Here, we present InCellCryst, an advanced pipeline for producing homogeneous microcrystals directly within living insect cells. We have demonstrated the pipeline on five different proteins (IMPDH, HEX-1, Cathepsin B, Luciferase and EGFP-µNS), representing a selection of soluble proteins of different source organisms that crystallize in insect cells in their native compartment or, in case of peroxisomes, readily in the cytoplasm or nucleus of the cells. Importantly, as shown for IMPDH and HEX-1, InCellCryst can produce crystals from native protein sequences, without purification tags or even remnants of proteolytically removed tags, within a quasi-native cellular environment. The rich source of biomolecules in the cellular environment allows the identification of native ligands by co-crystallization at quasi physiological conditions, representing a unique feature of InCellCryst.

The unmodified IMPDH (ori) as well as variants without the native (cyto) or with an artificial PTS1 motif crystallize within the cytosol, but no crystallization can be observed when the protein is translated into the ER. IMPDH crystallized with or without a PTS1 signal (peroxisomal import) in the cytosol, forming thick needles with a square base, similar to the unmodified version of the protein. The unit cell parameters of all IMPDH crystals remained unchanged as verified by SAXS-XRPD. All IMPDH structures show natural ligands at the canonical binding sites 1 and 2 in the Bateman domain. However, instead of guanosine monophosphate (GMP) found in the IMPDH N-His structure solved from isolated crystals, the structures solved in this study allow a clear identification of GDP in the canonical binding site 2, stabilized by hydrogen bonds to Lys133 and Arg101 that coordinate the α-phosphate and β-phosphate of GDP. In addition, a phosphate is bound to the IMP binding site of the catalytic domain of the IMPDH structures. As observed in the previously published IMPDH structure solved by SFX20, the canonical binding site 1 incorporates an ATP molecule. However, we observed two conformations of the bound ATP, where the gamma phosphates of the adjacent ATP molecules are either opposing or facing each other. We were able to identify naturally bound ligands and their conformations in the canonical nucleotide binding sites of the IMPDH ori and cyto structures, at a resolution of 2.3 and 2.4 Å, respectively. The second binding site is unambiguously occupied by GDP, instead of the previously proposed GMP20, demonstrating that crystal isolation and storage can alter the information obtained due to hydrolysis of the ligand.

>[2x]MGENTNLRTKTLRDGTTAEELFSQDGLSFNDFIILPGFIDFDSSKVNVSGQFTKNILLHLPLVSSPMDTVTESSMARAMALMGGIGVIHNNCTVEQQARMVRSVKLYRNGFIMKPKSVSPDVPVSTIRNIKSEKGISGILVTEGGKYDGKLLGIVCTKDIDFVKDASAPVSQYMTRRENMTVERYPIKLEEAMDVLNRSRHGYLPVLNDKDEVVCLCSRRDAVRARDYPNSSLDRNGHLLCAAATSTREADKGRVAALSEAGIDVLVLDSSQGNTIYQVSFIRWVKKTYPHLEVVAGNVVTQDQAKNLIDAGADSLRIGMGSGSICITQEVLACGRPQATAIYKVARYAASRGVPCVADGGLRNVGDVCKALAVGANVAMLGSMIAGTSETPGEYFFKDGMRLKGYRGMGSIDAMLQGRESGKRYLSENETLQVAQGVAGAVLDKGSVLKLLAYIHKGLQQSAQDIGEVSFDAIREKVYEGQVLFNRRSLTAQSEGAVHSLHHYERKLFAA> KLQEAHKLQEAHKLQEAH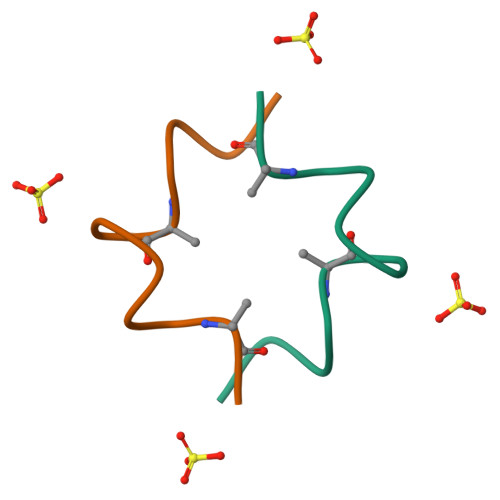KLQEAH3,8-bis(oxidanyl)-7-(piperidin-1-ylmethyl)-[1]benzofuro[3,2-c]chromen-6-one 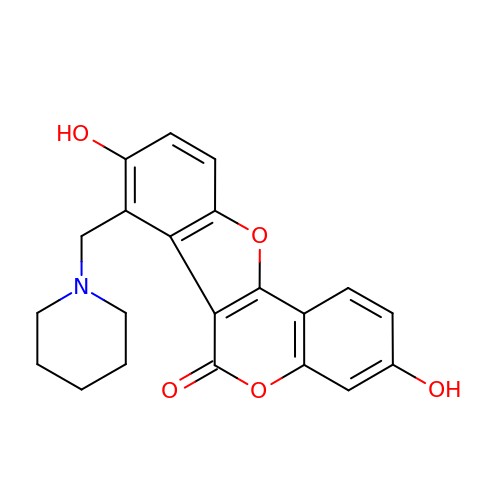| C21 H19 N O5 | SORWCEYAEWEEFV-UHFFFAOYSA-N>[3x]MASMERFLSVYDEVQAFLLDQLQSKYEIDPNRARYLRIMMDTTCLGGKYFRGMTVVNVAEGFLAVTQHDEATKERILHDACVGGWMIEFLQAHYLVEDDIMDGSVMRRGKPCWYRFPGVTTQCAINDGIILKSWTQIMAWHYFADRPF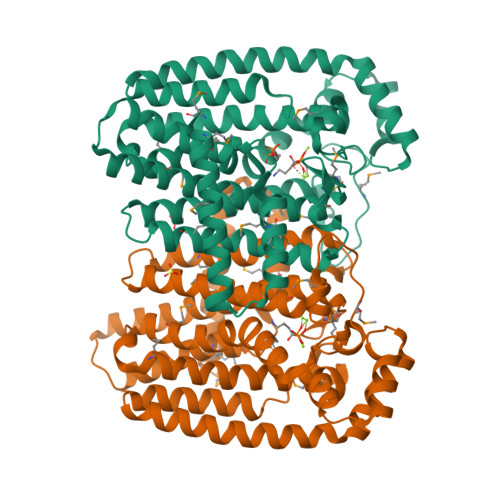LKDLLCLFQKVDYATAVGQMYDVTSMCDSNKLDPEVAQPMTTDFAEFTPAIYKRIVKYKTTFYTYLLPLVMGLFVSEAAASVEMNLVERVAHLIGEYFQVQDDVMDCFTPPEQLGKVGTDIEDAKCSWLAVTFLGKANAAQVAEFKANYGDKDPAKVAVVKRLYSEANLQADFAAYEAEVVREVESLIEQLKVKSPTFAESVAVVWEKTHKRKK>[2x]HHHHHHSSGLVPRGSHMAGLGNVTGAVASG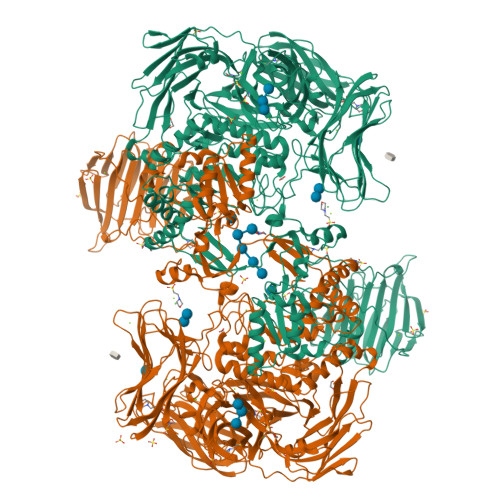DSLTLTLDNGTSASDILELDVLSEELLRVDYRPSGAAPSPSTPMIDPDASWDAVGATIDTSGDPIVVTTPRMRIEIARTPARMTIKKADGTTLLWEPASGGVFEDGVRFQRGSTDNIYGIRSFNAQEDVGGLLRNSSDHPAHAGQQGDAGGPFMWSTAGYGVLVDSDGGYPYTDTTGKLEFYYGGTPTEGRRYTKTNVEYYIMVGEPKEIMASYAQVTGTAPMLPKWSLGFMNFEWGIDQDELEAHVDGYRARNIPIDAFALDYDWMDYGEDNYGEFRWNTDNFPDAATTQLKEDMEAEGIRLIGIRKPRIITRDFANQRTQQYYDADSNGYFYPGHNEYTDYFIPVTVRSFDPYQQASRDWWWQHSIDAFDKGIVGWWNDETDKVDSGSAQYWFGNFSTGFTSQAMYDGQRDYTNDGVRVWQTARSYYPGAQRYATTLWSGDIGTQFYKGELFNWAPGMQEQPRIMLSSANLGQPKWGMDTGGFNSLGGASGPNPSPELYTRWMQFGAFTPVFRVHGNYNQQRQPWLYGATAEEASKAVMHTRYSLLPYMYAYEREASETGLGLIKPLLFDYPNDPQAADYTEAWMFGDWLLVSPVLGEAQHSKQIYLPAGTWIDYHRGQTYSGGQTIHYPVNADTWTDVPLFVKQGAIIPNQQVLDYVDQQSVTTVNVDIFPSASETSFTYYEDDGSSYDYESGSSFEQRLAAQDLSSSVRVEVGAGSGSYTPDVQHYVLKIHGRAGSAVTAGGSALTGYGDLQALQAASGSGWASGRDIYGDVTYVKLPAASGSATVVEVSGSAPSAATHAIYEVEDASRSGATPTTRAGINTNHSGYSGSGFVDKLDVPGAAVTVYANAPVSGDYPVELRYANGSGSAKTLSVYVNAARVQQLSLADTGAWSQWGTQTTTLPLTAGQNIITYKYDSDAGDTGGVNLDYIRVPFAPTQAEYAAESAKLWGGAGTSQDHWFYKGAAFVDNLTGVGAEASFDVYAPSAGTYNLSLRYANGTGSTKTLSAIVNGGAASTVTLTSPGMNWNLWNEHTMTATLTAGRNTISFRRNSGNSGNVNLDRLAVSASAITTLASERNLLDNGDFERDTTYNSNWTQWQPSGQPSAFGIDSGNALHPPEGPARRNQRAYFHSDNAYQQSIHQVVDVPVNNATYRLEAKVRMKNTTPTTARAEVQGHGGSPIYANISNDGVWKTIVIDNINVTSGSVDVGFYVDSPGYTTLHIDEVTLTRAP> GSMLIDAIHGAKMSTKLLVSLKV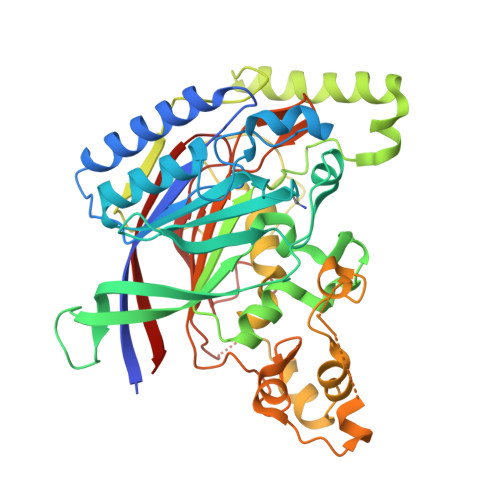LVIQLNPQIGQVDQTIKRTWSILDKVTKSATYVKPDIILFPEFALTGYSFHARKDILPYVTKKDEGPSFELAKSISEKFQCYTIIGYPEEDDEQKLYNSALVVNPQGGQIFNYRKTFLYDTEMNWDCEENPEGFQTFPMDFSKCAKLSNEDSYNRDVTLKASIGISMDLSPYKFMAPFNHFEFSSFCVDNNVELILCPMAWLNSTSITDKQTLHNNSLLEAAKNKIAFALKEQGLPLAGSQGIYQLKIGDSQRTPRVPSDDSTSEYKDMDEPDMSNVNYWILRFFPFLYFKLRINWFKNSSLIESILGKTRMPLDHEYYKDGKHKEDTIDLLDSEEVIKDTVLEKTFLGTSLGQPWKFQGKNAILVLANRCGTEDGTTIFAGSSGIYKFNGKKPKGSQDDDESSLDSLNESVELLGNLGKGLEGAILREVQFEVFR> SDTANAPFLCESEQLLIHPKEELSRNNSMVWIVNTKDYKQGVRIEKCLKRQLGKPCNFCDADTECKQLFHY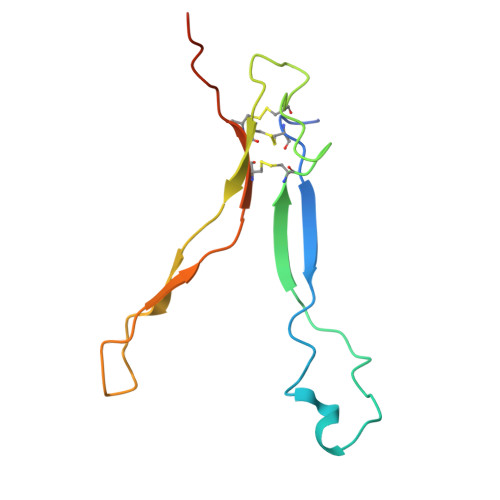RTLVAVDKVTKKPYKEQVLLPSCCKCAKILSTGWSHPQFEK> GPEFVSFANQLQALGLKLREVPGDGNCLFRALGDQLEGHSRNHLKHRQETVDYMIKQREDFEPFVEDDIPFEKHVASLAKPGTFAGNDAIVAFARNHQLNVVIHQLNAPLWQIRGTEKSSVRELHIAYRYGEHYDSVRRINDNSEAPAHLQTDFQMLHQD

Sixteen ovarian tumor (OTU) family deubiquitinases (DUBs) exist in humans, and most members regulate cell-signaling cascades. Biochemical analysis and five crystal structures of OTU DUBs with or without Ub substrates reveal four mechanisms of linkage specificity. Mechanistic and structural studies of three closely related, unstudied OTUs with distinct cleavage profiles revealed four mechanisms for achieving linkage specificity, namely (1) the use of additional Ub-binding domains (UBDs), (2) specific recognition of a ubiquitinated sequence, (3) the use of a conserved S1’ Ub-binding site on the OTU domain itself, and (4) the use of an S2 site enabling DUBs to bind longer chains in a linkage-specific manner. We selected three members of the OTUD family for additional investigation: the unstudied Lys63-specific OTUD1, the cdc48/p97 interactor OTUD2 that cleaves atypical linkages (Lys11, Lys27, Lys29, and Lys33), and OTUD3, another unstudied DUB with activity against Lys6- and Lys11-linked diUb.

To understand the specificity of OTUD domains at the molecular level, we determined high-resolution crystal structures of OTUD1 (aa 287–437, 2.1 Å), OTUD2 (aa 132–314, 1.5 Å), and OTUD3 (aa 52–209, 1.55 Å). The catalytic domains are structurally similar to each other and to OTUD5 (Huang et al., 2012) and S. cerevisiae Otu1 (yOtu1) (Messick et al., 2008), root-mean-square deviations (rmsds) being from 0.6–1.0 Å. Catalytic triads are in competent conformations, as observed for pOTUD5 in complex with a Ub suicide probe (Huang et al., 2012). UBDs do not always influence linkage specificity, at least for diUb substrates, as shown for OTUD3, where the removal of the UBA domain did not change its ability to cleave Lys6- and Lys11-linked diUb. Importantly, the amino acid sequence in the loops varies significantly between OTUD family members, in particular in the His and V loops, indicating changes that may account for the observed differences in linkage specificity. Substitution of the His loop of OTUD3 by the corresponding sequence in OTUD1 (mutating R178YGE to LSNG) rendered the protein significantly less active in comparison to the wild-type (WT) enzyme and affected its ability to target Lys11-linked, but not Lys6-linked, diUb, even at very high concentrations. Hence, we engineered an OTU domain with a unique specificity profile against diUb. Altogether, the structural and mutagenesis data revealed distinct S1’ Ub-binding sites on OTUD family enzymes that contribute to their ability to target selected Ub linkages. An additional enzyme worth studying is OTUD3, given that it is, so far, the only DUB that cleaves Lys6-linked diUb with some degree of specificity.> SSGW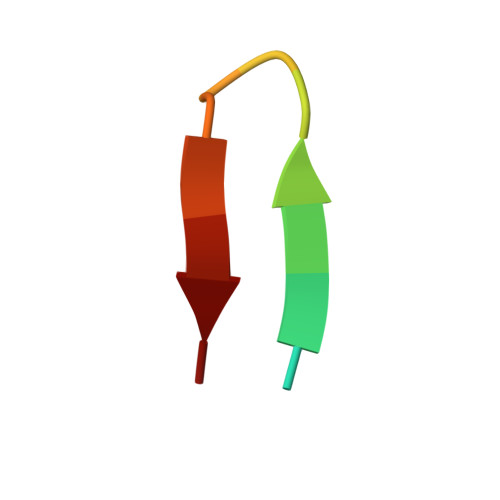MLDPIAGKWSR>MKLAVAGKGGVGKTTVAAGLIKIMASDYDKIYAVDGDPDSCLGQTLGLSIEEAYAITPLIEMKDEIREKTGDGGLLILNPKVDGDLDKYGRYIDDKIFLIRMGEIKKGGSQCYCRENSFLGSVVSALFLDKKEAVVMDMGAGIEHLTRGTAKAVDMMIAVIEPNLNSIKTGLNIEKLAGDLGIKKVRYVINKVRNIKEEKLIKKHLPEDKILGI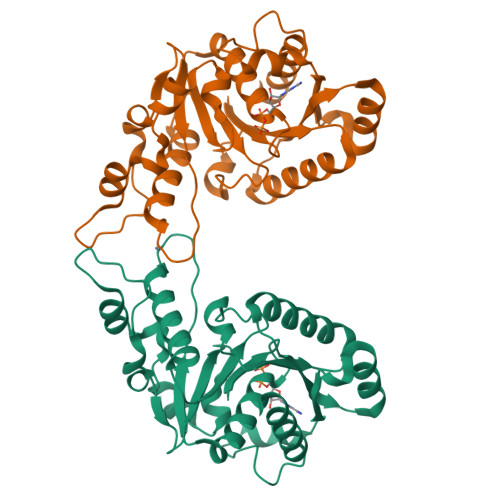IPYNELFIELSLKGEEIWQSTNPAFVNLHDIYQKLRLEVG[2x]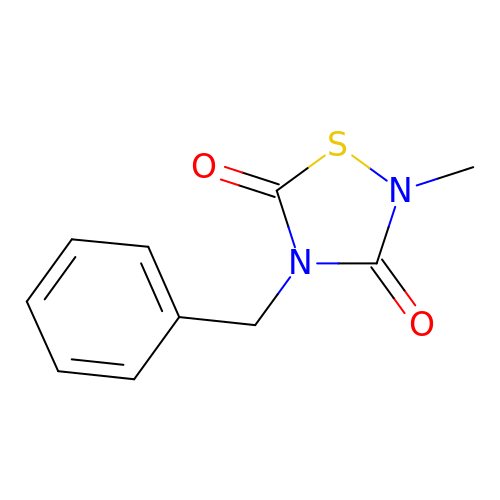2-methyl-4-(phenylmethyl)-1,2,4-thiadiazolidine-3,5-dione | C10 H10 N2 O2 S | JDSJDASOXWCHPN-UHFFFAOYSA-N> GUGUGCCCGGCAUGGGUGCAGUCUAUAGGGUGAGAGUCCCGAACUGUGAAGGCAGAAGUAACAGUUAGCCUAACGCAAGGGUGUCCGUGGCGACAUGGAAUCUGAAGGAAGCGGACGGCAAACCUUCGGUCUGAGGAACACGAACUUCAUAUGAGGCUAGGUAUCAAUGGAUGAGUUUGCAUAACAAAACAAAGUCCUUUCUGCCAAAGUUGGUACAGAGUAAAUGAAGCAGAUUGAUGAAGGGAAAGACUGCAUUCUUACCCGGGGAGGUCUGGAAACAGAAGUCAGGAGAAGUCAUAGUACCCUGUUCGCAGGGGAAGGACGGAACAAGUAUGGCGUUCGCGCCUAAGCUUGAACGGCCGUAUACCGAACGGUACGUACGGUCGUGUG;> GGGGUUAU

Group II introns are ubiquitous self-splicing ribozymes and retrotransposable elements evolutionarily and chemically related to the eukaryotic spliceosome, with potential applications as gene-editing tools. The site also harbors a metal-ion cluster formed by two divalent (M1–M2) and two monovalent (K1–K2) ions. In the first step of splicing, depending on whether the intron follows a hydrolytic or a transesterification mechanism, respectively, a water molecule or the 2′-OH group of a bulged adenosine in D6, activated by M2 and by the triple helix, attack the 5′-splice junction of the precursor (5e-I-3e), forming an intron/3′-exon intermediate (I-3e), in which the scissile phosphate (SP) is coordinated by K2. In the second step of splicing, the 5′-exon (5e), activated by M1, performs a nucleophilic attack on the 3′-splice junction, releasing ligated exons (5e-3e) and a linear or lariat form of the excised intron.

After incorporating the resulting triple base mutations (C289A/C358A/G385U, aka the A-mutant; C289G/C358G/G385C, aka the G-mutant; and C289U/C358U/G385A, aka the U-mutant), we monitored effects on splicing kinetics. First, we determined crystal structures of the G and U mutants in the presence of potassium and magnesium at 3.4 and 3.6 Å resolution, respectively. Importantly, both mutant structures adopt the triple-helical configuration that corresponds with that of the wild-type intron structure. The Fo − Fc simulated-annealing electron density omit maps calculated by omitting the J2/3 residues and the catalytic metal cluster reveal strong electron density signal for the triple helix conformer, as in wild type (total peak height for the nucleobase of G288 = 8.9 σ and 6.7 σ for the G and U mutants, respectively; maximum peak height for the metals = 9.5 σ and 6.6 σ for the G and U mutants, respectively; Fig. 2b). Moreover, the Fo − Fc maps calculated by omitting the first intron nucleotide (G1) show that the 5′-splice junction has undergone cleavage in both mutants during the crystallization process. In summary, the similarity of these mutant structures with that of wild type suggests that, despite some reductions in rate, the first step of splicing is structurally and mechanistically unaffected by the G and U mutations. Specifically, in the presence of near-physiological potassium and magnesium concentrations, the first splicing step of the G-mutant is ~12-fold slower and that of the U-mutant ~7-fold slower than in wild type. Moreover, the second splicing step of the G-mutant is ~48-fold slower and that of the U-mutant ~8-fold slower than in wild type. But when we replaced C358 with either a G or a U, the mutated intron accumulated linear I-3e intermediate, indicating a defect in the progression onto the second step of splicing.>GPGLKQKIVIKVAMEGNNCRSKAMALVASTGGVDSVALVGDLRDKIEV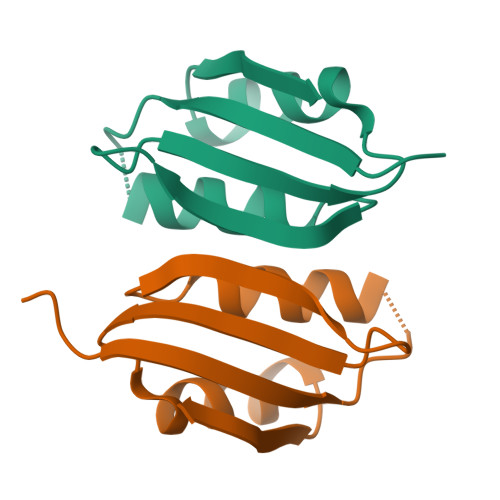VGYGIDPIKLISALRKKVGDAELLQVS[2x]7-[[(1R,2S)-2-azanylcyclohexyl]amino]-5-[[3-[(2S,6R)-2,6-dimethylmorpholin-4-yl]phenyl]amino]-4-oxidanylidene-3H-pyrido[3,4-d]pyridazine-8-carbonitrile 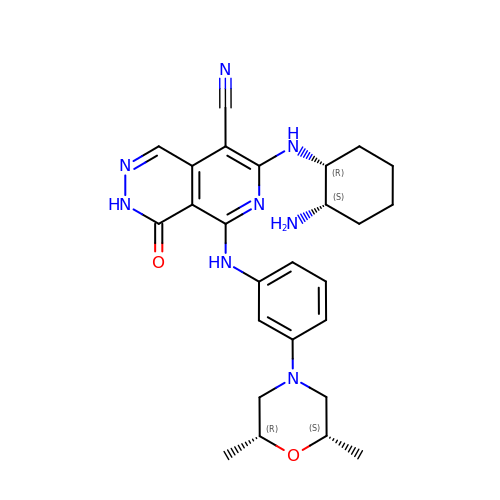| C26 H32 N8 O2 | KGWLGIOZFOBIIA-VYXDICFBSA-N> MPLSPPTNLHLEANPDTGVLTVSWERSTTPDITGYRITTTPTNGQQGNSLEEVVHADQSSCTFDNLSPGLEYNVSVYTVKDDKESVPISDTIIPEVPQLTDLSFVDITDSSIGLRWTPLNSSTIIGYRITVVAAGEGIPIFEDFVDSSVGYYTVTGLEPGIDYDISVITLINGGESAPTTLTQQTAVPPPTDLRFTNIGPDTMRVTWAPPPSIDLTNFLVRYSPVKNEEDVAELSISPSDNAVVL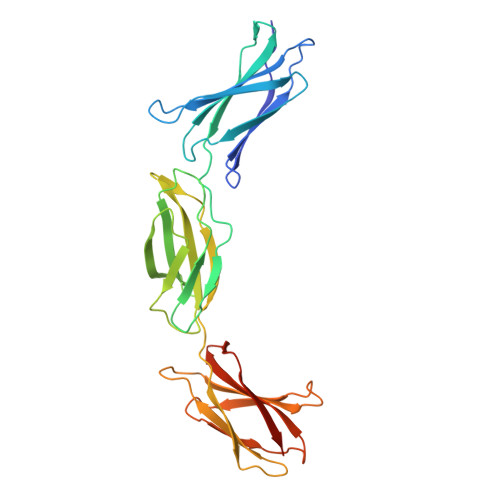TNLLPGTEYVVSVSSVYEQHESTPLRGRQKTGSAHHHHHH> PLGSEEEEEDAGLVAEAEAVAAGWMLDFLCLSLCRAFRDGRSEDFRRTRNSAEAIIHGLSSLTACQLRTIYICQFLTRIAAGKTLDAQFENDERITPLESALMIWGSIEKEHDKLHEEIQNLIKIQAIAVCMENGNFKEAEEVFERIFGDPNSHMPFKSKLLMIISQKDTFHS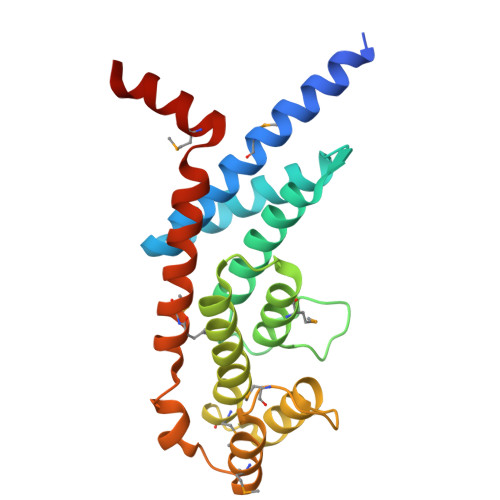FFQHFSYNHMMEKIKSYVNYVLSEKSSTFLMKAAAKVVESKR> MISKYRYLHCARKLVKQSVQAFGGGHHHHEYDWRDDPKVNKDIEEDIRDRGWHPETYDFPYTKKHDDWVFDVTMPSQNYQTDLTVNIHPENKKMHVMKQVMRQSYWDAEHDMAHEYDYESEDLDFQCESFKSQHFRKKGPISQYLILGLLPILYFGTEFFYNHYPDEDYWRVAHPPPLDYPDTDDTDDTETFKDYKSFTGRRMVDTGIVDPLWYDI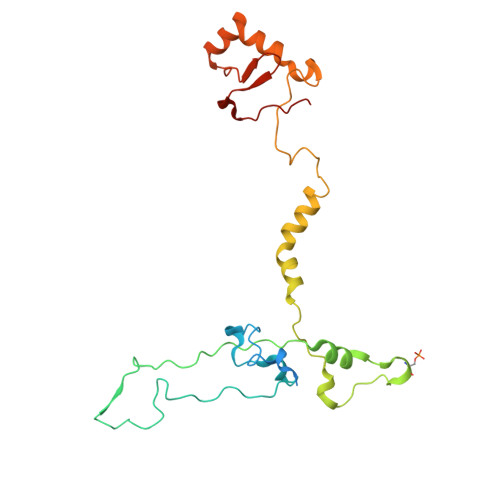REGKKVYYDWAGVNQPMEDI> F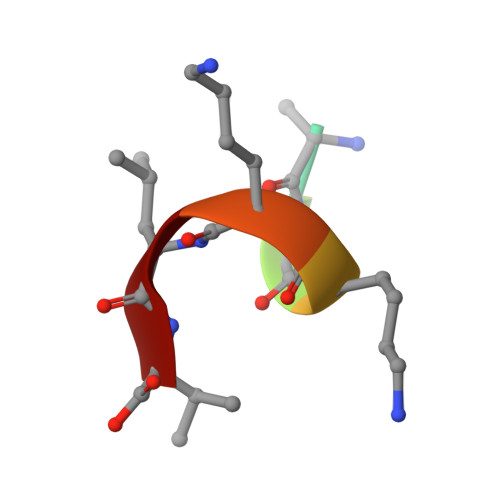EAKKLV>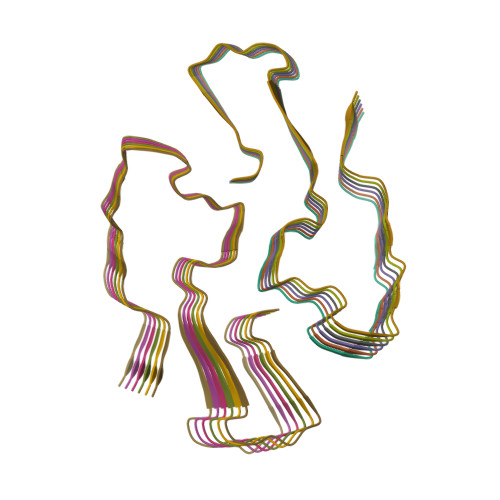SFFSFLGEAFDGARDMWRAYSDMREANYIGSDKYFHARGNYDAAKRGPGGVWAAEAISDARENIQR[12x]>MANLFKLGAENIFLGRKAATKEEAIRFAGEQLVKGGYVEPEYVQAMLDREKLTPTYLGESIAVPHGTVEAKDRVLKTGVVFCQYPEGVRFGEEEDDIARLVIGIAARNNEHIQ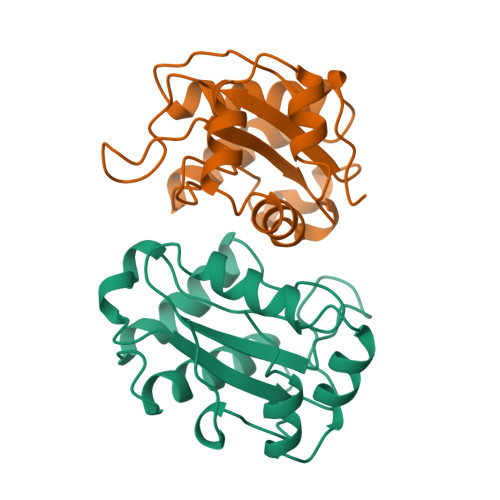VITSLTNALDDESVIERLAHTTSVDEVLELLAGRK[4x]> MGIVSQTRNKELLDKKIRSEIEAIKKIIAEFDVVKESVNELSEKAKTDPQAAEKLNKLIEGYTYGEERKLYDSALSK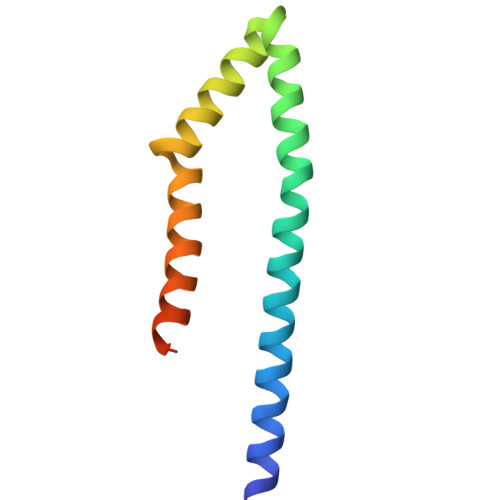IEKLIETLSPARSKSQST Breakdown is then initiated with the conversion of the C‐3 hydroxyl group to a ketone (cholest‐4‐en‐3‐one, cholestenone) by the oxidase ChoD, and further oxidation at the C‐26 “tail” region via a three‐step process involving oxidation to the hydroxyl, aldehyde, and carboxylic acid species. These sidechain‐modifying reactions are catalysed by the cytochromes P450 CYP125A1 and CYP142A1 (CYP125 and CYP142 hereafter). Comparison of the effect of complementing a CYP125 knockout in the CDC1551 strain of Mtb (which does not express the CYP142 protein), with CYP125 or CYP142 reveals that the two enzymes are functionally redundant with respect to growth on cholesterol. Here we present a series of compounds based on an ethyl 5‐(pyridin‐4‐yl)‐1H‐indole‐2‐carboxylate pharmacophore which bind strongly to both Mtb cholesterol oxidases CYP125 and CYP142.

Examination of the overlap of the co‐crystal structures for compounds 1–3 in CYP125 show that the incorporation of a five membered ring onto the phenyl ring offers a vector for further elaboration. This led to the development of compound 4, where the pyridyl ring is fused onto the 5‐position of an indole ring. The indole ring has an ethoxycarbonyl group in the 2‐position and, along with the NH of the indole, provide vectors for further elaboration. The affinity (KD) of compound 4 was shown to be 3.0 μM (CYP125) and 0.75 μM (CYP142), an improvement in affinity in comparison to the original fragment hits. Gratifyingly, the CYP125 binding mode is preserved when these fragments are merged and modified to develop compound 4. Although compound 4 is similarly effective in bridging the hydrophobic active site regions in both CYP125 and CYP142, the observed pose is notably different. In CYP125, compound 4 extends perpendicular above the heme and the indole occupies a small pocket formed by Val267, Glu271, Trp414, and Leu415 which is not utilized by cholestenone (PDB code: 2X5 W). In both CYP125 and CYP142 the indole nitrogen in compound 4 forms solvent‐mediated polar interactions. In CYP125 this involves a water molecule coordinated between the carboxyl oxygen of Met200, and the sidechain of Glu271, and for CYP142, the interaction occurs with an acetate ion derived from the crystallisation solution. Combining information from the binding position of compound 4 in both CYP125 and CYP142 suggested that elaboration of the compound from the indole nitrogen offered opportunities to exploit the space above Trp414 and Leu415 (CYP125), or the pocket surrounded by Ile65, Asp77, and Leu72 (CYP142) to further improve affinity.

>NGPSPNLPPGFDFTDPAIYAERLPVAEFAELRSAAPIWWNGQDPGKGGGFHDGGFWAITKLNDVKEISRHSDVFSSYENGVIPRFKNDIAREDIEVQRFVMLNMDAPHHTRLRKIISRGFTPRAVGRLHDELQERAQKIAAEAAAAGSGDFVEQVSCELPLQAIAGLLGVPQEDRGKLFHWSNEMTGNEDPEYAHIDPKASSAELIGYAMKMAEEKAKNPADDIVTQLIQADIDGEKLSDDEFGFFVVMLAVAGNETTRNSITQGMMAFAEHPDQWELYKKVRPETAADEIVRWATPVTAFQRTALRDYELSGVQIKKGQRVVMFYRSANFDEEVFQDPFTFNILRNPNPHVGFGGTGAHYCIGANLARMTINLIFNAVADHMPDLKPISAPERLRSGWLNGIKHWQVDYTGRCPVA[3x]>GSADLAHGGQVFSANCAACHLGGRNVVNPAKTLQKADLDQYGMASIEAITTQVTNGKGAMPAFGSKLSADDIADVASYVLDQSEKGWQG[2x]

Cyt c6 is a small, water-soluble protein (~12 kDa) that contains a heme group as its active center. As an essential electron carrier, Cyt c6 mediates between the cytochrome b6f complex and photosystem I (PSI), enabling electron transfer that is fundamental for sustaining photosynthesis by maintaining the continuous flow of electrons through the photosynthetic chain. The crystal structures of Cyt c6 from both species revealed a conserved fold, consisting of five α-helices, a bound heme group, and loop regions, which closely resembled previously characterized Cyt c6 proteins from other species. The heme was covalently linked to two cysteine residues via thioether bonds, and the central iron atom was axially coordinated by methionine and histidine residues, maintaining consistent coordination geometry in both oxidized and reduced states.

The reduced Cyt c6 proteins were generated using β-mercaptoethanol, while oxidized forms were prepared by adding potassium ferricyanide. Minimal differences were observed between the reduced and oxidized forms, with an RMSD of 0.446, indicating that heme coordination remains stable throughout redox transitions, consistent with the previous report. Structural comparisons between red-Cyt c6-7942 and oxi-Cyt c6-7942 revealed some differences in surface amino acids, particularly charged residues, despite the largely similar positions of heme-binding pocket residues. Analysis of the RMSD values for each residue between the oxidized and reduced forms of Cyt c6-7942 reveals some flexibility in the side chains of residues located on the protein surface, including Gln8, Arg22, Glu45, Thr48, Lys64, and Glu82. However, noticeable differences in the surface potential map are observed near the acidic patch (Asp68, Asp69, Asp72, and Asp2 in Cyt c6-7942), which can be attributed to the flexibility of the N-terminus. Additionally, the oxidized and reduced forms of Cyt c6-7942 exhibited highly consistent dimeric interactions. Small structural differences between red-Cyt c6-7942 and oxi-Cyt c6-7942 suggest insights into the functional mechanism of photosynthetic electron transfer. In contrast, the oxidized form undergoes structural adjustments to accommodate the oxidized heme, providing the flexibility required for efficient electron transfer and subsequent dissociation from PSI. This rapid structural transition may facilitate flexible and effective electron transfer through Cyt c6.> MGHHHHHHMSHTILLVQPTKRPE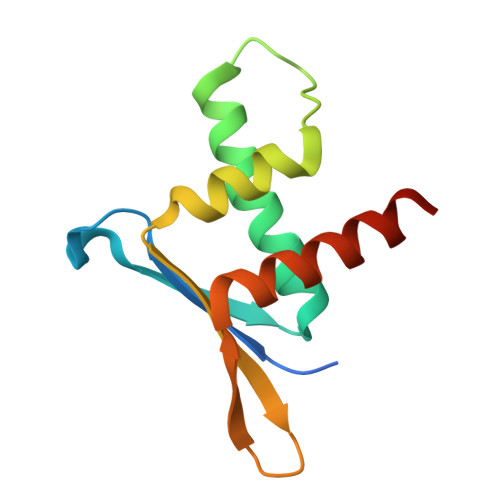GRTYADYESVNECMEGVCKMYEEHLKRMNPNSPSITYDISQLFDFIDDLADLSCLVYRADTQTYQPYNKDWIKEKIYVLLRRQAQQAGK> MGAQVST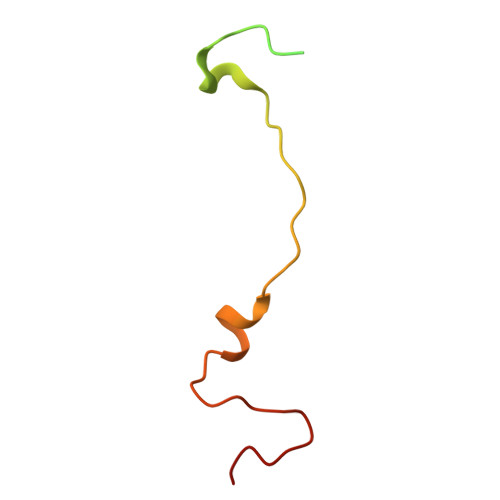QKSGSHENQNILTNGSNQTFTVINYYKDAASSSSAGQSFSMDPSKFTEPVKDIMLKGAPALN The packaging of cargo transmembrane proteins into COPII-coated vesicles entails a direct interaction between COPII protein and cytoplasmically-oriented ER export signals. About a half dozen export signals have been identified to date, almost all comprising short peptide motifs, all of them binding to the Sec24 subunit of the COPII inner coat. The ΦC export signal was identified in studies of p24-family and ERGIC-53 proteins, and comprises a C-terminal signature of a pair of hydrophobic residues or a single terminal valine residue. The ΦC motif contacts a site on Sec24a that is also the binding site for the LxxLE- and DxE-class export motifs (Miller et al., 2003; Mossessova et al., 2003).

A series of ΦC-signal peptides was synthesized, based on a core sequence of yeast Emp24p, and individual peptides were soaked at high concentrations into two crystal forms of human COPII protein: one comprising Sec23a/Sec24a•Sec22b, the other Sec24c. For all ΦC sequences, we observed clear evidence for peptide binding to a site on Sec24a in the Sec23a/Sec24a•Sec22b crystals, based on the presence of residual electron density that matches the peptide sequence (this binding site is occluded in the Sec24c crystals). (C) Residual (Fo-Fc) electron density (2.6 Å resolution, 2.6 σ contour) for a bound ΦC peptide containing the terminal Val-Val motif of human p24β1. Thus, specific recognition of the ΦC motif involves the terminal carboxylate group bonding to Arg750 and Arg752 of Sec24a, with the penultimate hydrophobic residue of the motif nestling against Tyr496, and the terminal hydrophobic residue fitting to a pocket of hydrophobic side chains.

> MTTYLEFIQQNEERDGVRFSWNVWPSSRLEATRMVVPVAALFTPLKERPDLPPIQYEPVLCSRTTCRAVLNPLCQVDYRAKLWACNFCYQRNQFPPSYAGISELNQPAELLPQFSSIEYVVLRGPQMPLIFLYVVDTCMEDEDLQALKESMQMSLSLLPPTALVGLITFGRMVQVHELGCEGISKSYVFRGTKDLSAKQLQEMLGLSKVPLTQATRGPQVQQPPPSNRFLQPVQKIDMNLTDLLGELQRDPWPVPQGKRPLRSSGVALSIAVGLLECTFPNTGARIMMFIGGPATQGPGMVVGDELKTPIRSWHDIDKDNAKYVKKGTKHFEALANRAATTGHVIDIYACALDQTGLLEMKCCPNLTGGYMVMGDSFNTSLFKQTFQRVFTKDMHGQFKMGFGGTLEIKTSREIKISGAIGPCVSLNSKGPCVSENEIGTGGTCQWKICGLSPTTTLAIYFEVVNQHNAPIPQGGRGAIQFVTQYQHSSGQRRIRVTTIARNWADAQTQIQNIAASFDQEAAAILMARLAIYRAETEEGPDVLRWLDRQLIRLCQKFGEYHKDDPSSFRFSETFSLYPQFMFHLRRSSFLQVFNNSPDESSYYRHHFMRQDLTQSLIMIQPILYAYSFSGPPEPVLLDSSSILADRILLMDTFFQILIYHGETIAQWRKSGYQDMPEYENFRHLLQAPVDDAQEILHSRFPMPRYIDTEHGGSQARFLLSKVNPSQTHNNMYAWGQESGAPILTDDVSLQVFMDHLKKLAVSSA;> EGLRVVNLLQERNMLPSTPLKPPVPNLHEDIQKLNCNPELFRCTLTSIPQTQALLNKAKLPLGLLLHPFKDLVQLPVVTSSTIVRCRSCRTYINPFVSFLDQRRWKCNLCYRVNDVPEEFLYNPLTRVYGEPHRRPEVQNATIEFMAPSEYMLRPPQPPVYLFVFDVSHNAVETGYLNSVCQSLLDNLDLLPGNTRTKIGFITFDSTIHFYGLQESLSQPQMLIVSDIEDVFIPMPENLLVNLNESKELVQDLLKTLPQMFTKTLETQSALGPALQAAFKLMSPTGGRMSVFQTQLPTLGVGALKPREEPNHRSSAKDIHMTPSTDFYKKLALDCSGQQVAVDLFLLSGQYSDLASLGCISRYSAGSVYYYPSYHHQHNPVQVQKLQKELQRYLTRKIGFEAVMRIRCTKGLSIHTFHGNFFVRSTDLLSLPNVNPDAGYAVQMSVEESLTDTQLVSFQSALLYTSSKGERRIRVHTLCLPVVSTLNDVFLGADVQAISGLLANMAVDRSMTASLSDARDALVNAVIDSLSAYRSSVLSNQQPGLMVPFSLRLFPLFVLALLKQKSFQTGTNARLDERIFAMCQVKNQPLVYLMLTTHPSLYRVDNLSDEGALNISDRTIPQPPILQLSVEKLSRDGAFLMDAGSVLMLWVGKNCTQNFLSQVLGVQNYASIPQPMTDLPELDTPESARIIAFISWLREQRPFFPILYVIADESPMKANFLQNMIEDRTESALSYYEFLLHIQQQVNK;> MVLLTMIARVADGLPLAASMQEDEQSGRDLQQYQSQAKQLFRKLNEQSPTRCTLEAGAMTFHYIIEQGVCYLVLCEAAFPKKLAFAYLEDLHSEFDEQHGKKVPTVSRPYSFIEFDTFIQKTKKLYIDSRARRNLGSINTELQDVQRIMVANIEEVL;> VTSVV> APYASLTEIEHLVQSVCKSYRETCQLRLEDLLRQRSNIFSREEVTGYQRKSMWEMWERCAHHLTEAIQYVVEFAKRLSGFMELCQNDQIVLL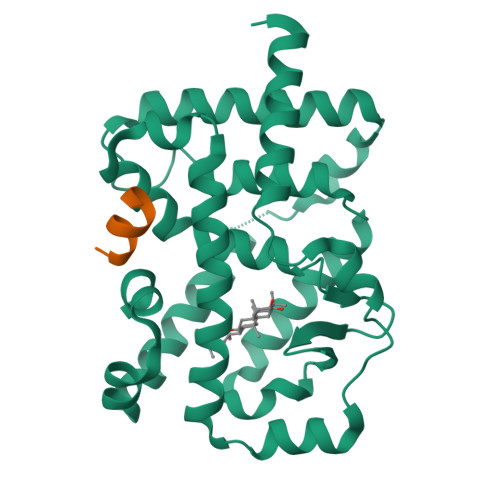KAGAMEVVLVRMCRAYNADNRTVFFEGKYGGMELFRALGCSELISSIFDFSHSLSALHFSEDEIALYTALVLINAHRPGLQEKRKVEQLQYNLELAFHHHLCKTHRQSILAKLPPKGKLRSLCSQHVERLQIFQHLHPIVVQAAFPPLYKELFS;> KHKILHRLLQDSS(4R)-4-[[(2S)-2-[[(2R)-2-[(2R,3S,4R,5R,6R)-5-acetamido-2-(hydroxymethyl)-3,6-bis(oxidanyl)oxan-4-yl]oxypropanoyl]amino]propanoyl]amino]-5-azanyl-5-oxidanylidene-pentanoic acid | C19 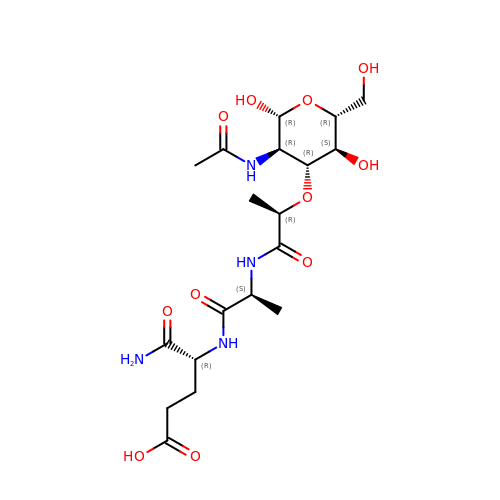H32 N4 O11 | BSOQXXWZTUDTEL-ZUYCGGNHSA-N>MAARGGRSEPPQLAEYSCSYTVSRPVYSELAFQQQRERRLPERRTLRDSLARSCSCSRKRAFGVVKTLLPILDWLPKYRVKEWLLSDIISGVSTGLVGTLQGMAYALLAAVPVQFGLYSAFFPILTYFVFGTSRHISVGPFPVVSLMVGSVVLSMAPDDHFLVPSGNGSALNSTTLDTGTRDAARVLLASTLTLLVGIIQLVFGGLQIGFIVRYLADPLVGGFTTAAAFQVLVSQLKIVLNVSTKNYNGILSIIYTLIEIFQNIGDTNIADFIAGLLTIIVCMAVKELNDRFKHRIPVPIPIEVIVTIIATAISYGANLEKNYNAGIVKSIPSGFLPPVLPSVGLFSDMLAASFSI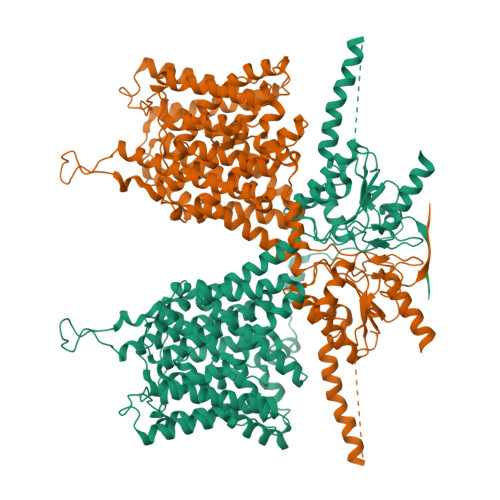AVVAYAIAVSVGKVYATKHDYVIDGNQEFIAFGISNVFSGFFSCFVATTALSRTAVQESTGGKTQVAGLISAVIVMVAIVALGRLLEPLQKSVLAAVVIANLKGMFMQVCDVPRLWKQNKTDAVIWVFTCIMSIILGLDLGLLAGLLFALLTVVLRVQFPSWNGLGSVPSTDIYKSITHYKNLEEPEGVKILRFSSPIFYGNVDGFKKCINSTVGFDAIRVYNKRLKALRRIQKLIKKGQLRATKNGIISDIGSSNNAFEPDEDVEEPEELNIPTKEIEIQVDWNSELPVKVNVPKVPIHSLVLDCGAVSFLDVVGVRSLRMIVKEFQRIDVNVYFALLQDDVLEKMEQCGFFDDNIRKDRFFLTVHDAILHLQNQVKSREGQDSLLETVARIRDCKDPLDLMEAEMNAEELDVQDEAMRRLAS[2x]> MAAASTYTENNILNALLRGVAFPLPAKTYVSLHTGDPGVGAGANEVSLSNWPAYVRREAEQGGAIGSGWTPAASGQTSNVNQLTYPANNGVAAVTVTHYAVFDAPTGGNLLFKAPLTVAR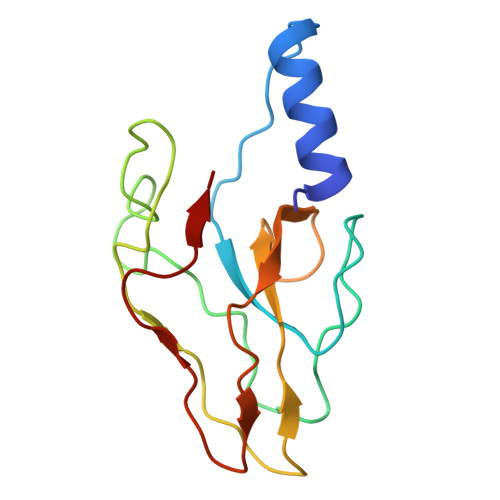TLQVGDVFVFDVGSLTAQAS>[12x]MLRTMLKSKIHRATVTCADLHYVG;>[12x]XVTIDADLMDAADLLEGEQVTIVDIDNGARLVTYAITGERGSGVIGINGAAAHLVHPGDLVILIAYATMDDARARTYQPRIVFVDAYNKPIDMGHDPAFVPENAGELLDPRLGVGLEHHHHHH

Here, we present biochemical and structural evidence that POA inhibits Mtb PanD in a competitive fashion and that it binds with a high degree of complementarity to the active site of the enzyme. PanD is a proenzyme and in the structure, we observed the processed active enzyme after cleavage between Gly24 and Ser25, and modification of Ser25 to a pyruvoyl group (Pyr25). The active protein consists of a β chain (Met1-Gly24) and an α chain (Pyr25 to ILE115). Our results show that resistance to PZA in PanD mutants primarily comes from alterations in two loops covering the active site that have subtle, but significant effects on the affinity and residence time of POA on the enzyme rather than from directly affecting POA binding interactions.

We also tested PZA, nicotinic acid (NA), and two POA analogs with chlorine atom at the 5-(para) or 6-(meta) position. None of these compounds inhibited Mtb PanD at concentrations up to 20 mM, except 6-Cl-POA which was also competitive and slightly less potent compared to POA (Ki = 1.00 (0.04) mM, Fig. 1c). The ITC data fit to a single-site model, with a Kd for POA of 0.71 (0.03) mM (n = 5) and that of 6-Cl-POA as 1.09 (0.04) mM (n = 3). The molecular surface of the active site indicated there was room to add a substituent to the pyrazine ring of POA at the 6-position based on the pose we selected. This was consistent with the finding that 6-Cl POA was an inhibitor of PanD and 5-Cl POA showed no inhibition. We cocrystallized Mtb PanD with the 6-Cl POA analog and refined the structure to 2.25 Å. A polder OMIT map showed clear electron density for the 6-Cl and it was oriented with the pyrazine ring in the same orientation as we fit POA. The POA binding pocket is relatively small (206 Å3) and not easily accessible, as there is only a narrow tunnel leading from the active site to the inside barrel of the PanD tetramer. With a diameter of ~3.4 Å, neither the substrate nor inhibitor could pass through the tunnel. The chlorine atom of 6-Cl-POA resides in this tunnel.>[2x]TASSVLLHTGQKMPLIGLGTWKSEPGQVKAAIKHALSAGYRHIDCASVYGNETEIGEALKESVGSGKAVPREELFVTSKLWNTKHHPEDVEPALRKTLADLQLE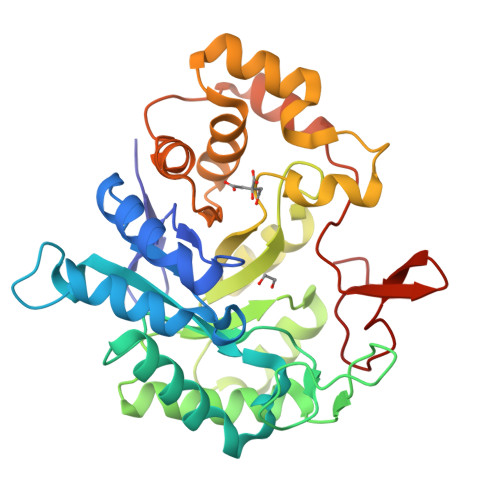YLDLYLMHWPYAFERGDNPFPKNADGTVRYDSTHYKETWKALEVLVAKGLVKALGLSNFNSRQIDDVLSVASVRPAVLQVECHPYLAQNELIAHCHARGLEVTAYSPLGSSDRAWRHPDEPVLLEEPVVLALAEKHGRSPAQILLRWQVQRKVICIPKSINPSRILQNIQVFDFTFSPEEMKQLDALNKNWRYIVPMITVDGKRVPRDAGHPLYPFNDPY> MVDGNYSVASNVMVPMRDGVRLAVDLYRPDADGPVPVLLVRNPYDKFDVFAWSTQSTNWLEFVRDGYAVVIQDTRGLFASEGEFVPHVDDEADAEDTLSWILEQAWCDGNVGMFGVSYLGVTQWQAAVSGVGGLKAIAPSMASADLYRAPWYGPGGALSVEALLGWSALIGTGLITSRSDARPEDAADFVQLAAILNDVAGAASVTPLAEQPLLGRLIPWVIDQVVDHPDNDESWQSISLFERLGGLATPALITAGWYDGFVGESLRTFV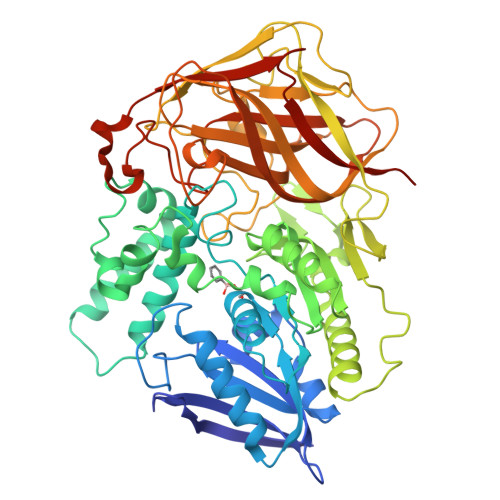AVKDNADARLVVGPWSHSNLTGRNADRKFGIAATYPIQEATTMHKAFFDRHLRGETDALAGVPKVRLFVMGIDEWRDETDWPLPDTAYTPFYLGGSGAANTSTGGGTLSTSISGTESADTYLYDPADPVPSLGGTLLFHNGDNGPADQRPIHDRDDVLCYSTEVLTDPVEVTGTVSARLFVSSSAVDTDFTAKLVDVFPDGRAIALCDGIVRMRYRETLVNPTLIEAGEIYEVAIDMLATSNVFLPGHRIMVQVSSSNFPKYDRNSNTGGVIAREQLEEMCTAVNRIHRGPEHPSHIVLPIIKRPLEHHHHHH2-(1-{[2-(2H-indazol-4-yl)-4-(morpholin-4-yl)pyrido[3,2-d]pyrimidin-6-yl]methyl}piperidin-4-yl)propan-2-ol | C27 H33 N7 O2 | 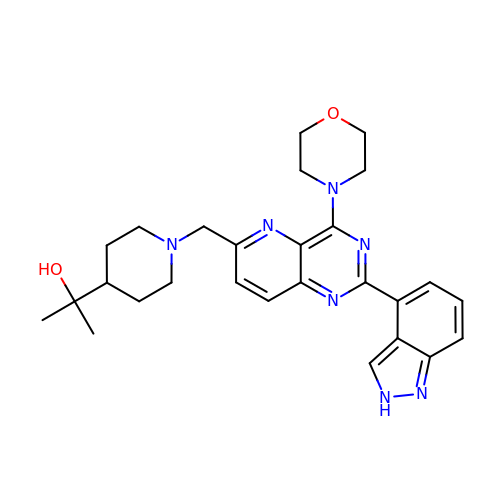YEOXTSXBPMKEQR-UHFFFAOYSA-N> SPEIMKDLSINFGKALDTCKKELDLPDSINEDFYKFWKEDYEITNRLTGCAIKCLSEKLEMVDADGKLHHGNAREFAMKHGADDAMAKQLVDLIHGCEKSIPPNDDRCMEVLSIAMCFKKEIHNLKWAPNMEVVVGEVLA

A primary pheromone-binding protein (PBP) from A. transitella, (AtraPBP1) has been identified based on its expression profile in male antennae and its biochemical properties. Understanding the structural basis of pheromone detection and elucidating the mechanisms of action of olfactory proteins will aid in the development of novel and stable mimics of one or more of the attractants. These pathways are mediated in part by pheromone-binding proteins (PBPs), which are believe to be important in solubilizing the hydrophobic ligands and serve as an initial transporter that present odorants to a receptor in the membrane to elicit an olfactory response. To answer these questions and to pave the way for the design of a stable synthetic sex pheromone useful as a mating disruptor, we solved the high-resolution crystal structures at high pH of the liganded AtraPBP1 complexed separately with the major constituent of the sex pheromone of A. transitella, (11Z,13Z)-hexadecadienal (Z11Z13-16Ald) and the secondary constituent, (11Z,13Z)-hexadecadienol (Z11Z13-16OH). The pH 6.5 AtraPBP1 structure complexed with either Z11Z13-16OH or Z11Z13-16Ald adopts the same core canonical fold described previously for pheromone-binding proteins consisting of six α-helices connected by loops.

The binding site is highly complementary to these linear molecules in this particular conformation and is unlikely to be capable of binding molecules, which are longer or significantly diverge in shape. Both pheromones are firmly stabilized into the binding pocket primarily by an array of hydrophobic interactions. The hydrophobic interactions are mediated by the side-chains of Leu8, Ile52, Met61, Leu68, Ileu94, Val111 and Ile114 that make numerous interactions with the carbon chain. In addition, a stacked arrangement of a quartet of phenylalanines at positions 12, 36, 76 and 118 interact with the ligands near the desaturated carbons. In the case of the Z11Z13-16Ald pheromone constituent, the oxygen of the aldehyde group is hydrogen-bonded to the positively charged Arg107 guanidinium group. In addition, two water-mediated hydrogen bonds with the backbone oxygen of both Met61 and Gly66 complete the binding mesh of Z11Z13-16Ald in AtraPBP1. Accordingly, they are both almost completely sequestered from the solvent by the protein (2.7% and 2.2% solvent accessibility for the alcohol and aldehyde forms respectively). The average B-factor for both structures is relatively low with 18.2 Å2 (holo Z11Z13-16Ald) and 13.0 Å2 (holo Z11Z13-16OH) respectively. Possible x-ray radiation-induced damage was found in the Z11Z13-16Ald bound structure at the early stages of the refinement consisting of an unambiguous, discontinuous 2Fo-Fc electron density at 1.14 Å resolution located where the disulfide bond between Cys19 and Cys54 should be. The same bond was found intact on the refined structure from a preliminary dataset collected on a home source at 1.54 Å using the same crystal (data not shown).>SNAMSEANSGPGRVTREQRGHLFLIGLDRAGKRNAFDSAMLADLALAMGEYERSEESRCAVLFAHGEHFTAGLDLMELAPKLAASGFRYPDGGVDPWGVVQPRRSKPLVVAVQGTCWTAGIELMLNADIAVAARGTRFAHLEVLRGIPPLGGSTVRFP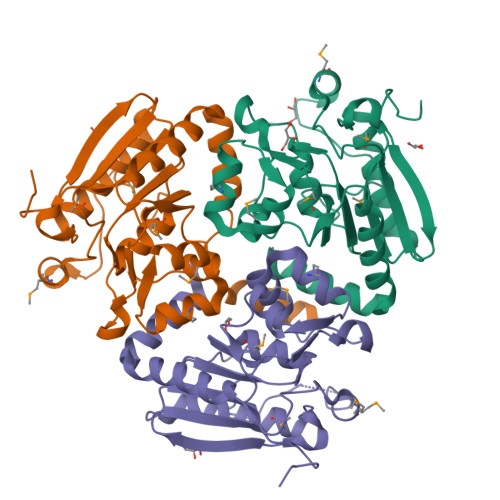RAAGWTDAMRYILTGDEFDADEALRMRLLTEVVEPGEELARALEYAERIARAAPLAVRAALQSAFQGRDEGDDAALSRVNESLAALIGSEDVREGVLAMV[3x]> GDPHMSEVITITKRNGAFQNSSNLSYNNTGISDDENDEEDIYMHDVNSASKSESDSQIVTPGELVTDDPIWMRGHGTYFLDNMTYSSVAGTVSRVNRLLSVIPLKGRYAPETGDHVVGRIAEVGNKRWKVDIGGKQHAVLMLGSVNLPGGILRRKSESDELQMRSFLKEGDLLNAEVQSLFQDGSA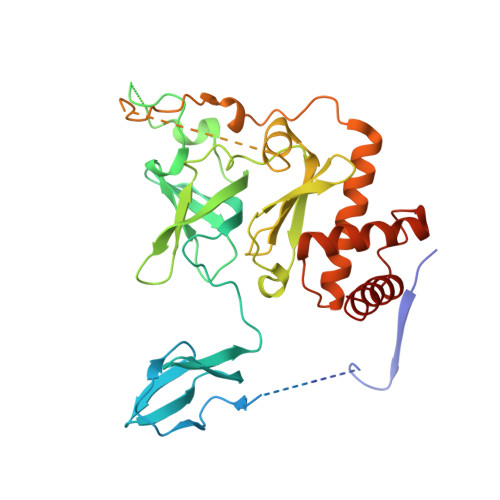SLHTRSLKYGKLRNGMFCQVPSSLIVRAKNHTHNLPGNITVVLGVNGYIWLRKTSQMDLARDTPSANNSSSIKSTGPTGAVSLNPSITRLEEESSWQIYSDENDPSISNNIRQAICRYANVIKALAFCEIGITQQRIVSAYEASMVYSNVGELIEKNVMESIGSDILTAEKMRGNGN> MGSDKIHHHHHHMAVNRFRLENGKEELALYQIQLLKDQSHNENEEDKVSSSSFRQRILGNLLQPPNERPELPSGLYVLGLTGISGSGKSSVAQRLKNLGAYIIDSDHLGHRAYAPGGP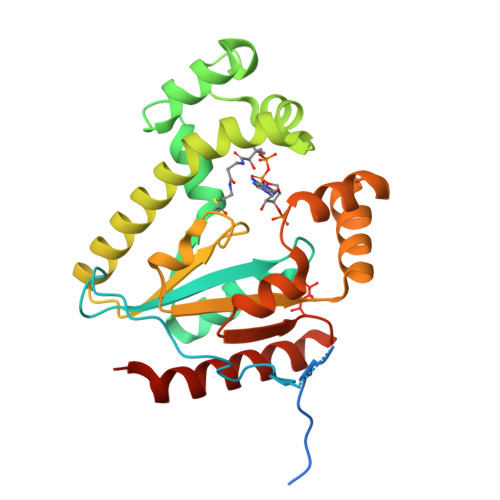AYQPVVEAFGTDILHKDGTINRKVLGSRVFGNKKQMKILTDIVWPVIAKLAREEMDVAVAKGKTLCVIDAAMLLEAGWQSMVHEVWTVVIPETEAVRRIVERDGLSEAAAQSRLQSQMSGQQLVEQSNVVLSTLWESHVTQSQVEKAWNLLQKRLPKAYQTRN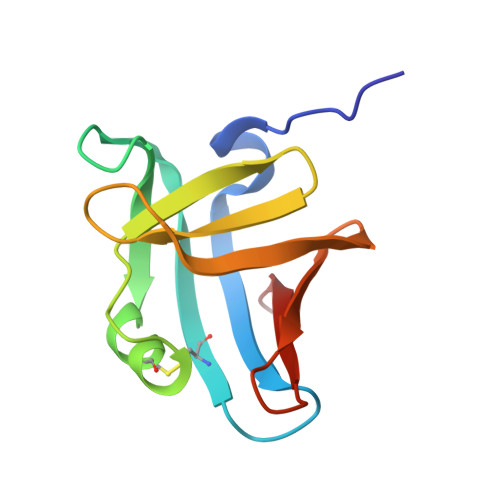> SSLILLSASDLAGQWTLQQDEAPAICHLELRDSEVAEASGYDLGGDTACLTRWLPSEPRAWRPTPAGIALLERGGLTLMLLGRQGEGDYRVQKGDGGQLVLRRATP> MRYTARFLDQTTGPHKAYKYTYMPDPRKLAPIE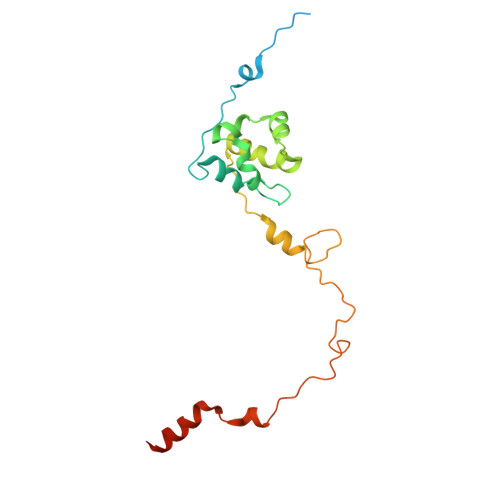TSMRSEVLPVVIRPPTSYVPNHEVFLEKADVHRLAPTSDFKATFKDWNDLMTCSKRELRTRGVPLLTRRAIRAAVLAFQNGNPPERFDTKEEWLYYKQFKTKDYSYRVVPELPEKYRPHQNGIDQAPVPNYGEINQMPQWAVEEEKRLTGKISAASK>[3x]MTDNKRPQLKDKEPAAKPARTRKPKNETVALVVEATTEAEAK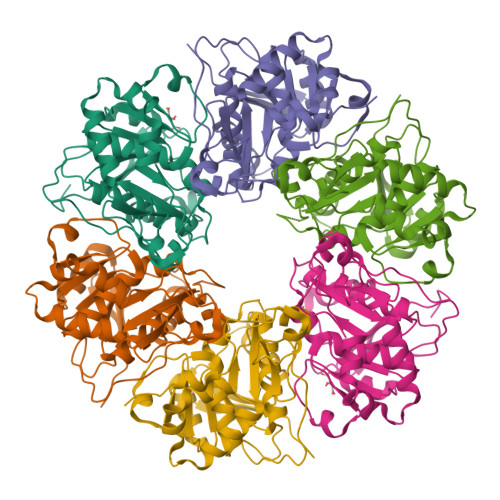KSLREGGLVPAAHEIMIPVGNMILAVDTQVLDKCALALAASDDPGRWFAENESLIHSTVFAPVAKGLHRVYPLLSVRPEVPAGYEASWPTQDHMPGLHLVVGGTGAGKSSYLASQDLTLVIRWGEPAERFDVEGATHAVSDLNEALAVAFVMARAGYRPAIDSFRNLVFGIESAAGEGGISTALYSAMTAINNVCSRLGIVVMVVVNPMATEAKAELVYNNMAASVAGMTVLMDGAVSKQTVRTLSGRT> DLPIAR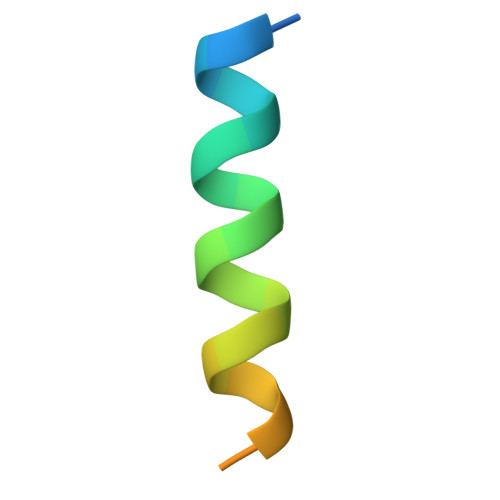RKSLQRFLEKRKERLVSTSPY>[4x]SSSVVLDSENGVETESRKLPSS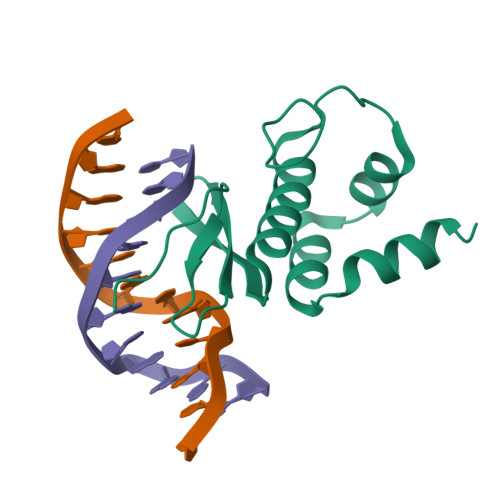KYKGVVPQPNGRWGAQIYEKHQRVWLGTFNEEEEAASSYDIAVRRFRGRDAVTNFKSQVDGNDAESAFLDAHSKAEIVDMLRKHTYADEFEQSRRKFVNG>[2x]MLLLTPGPTPIPERVQKALLRPMRGHLDPEVLRVNRAIQERLAALFDPGEGALVAALAGSGSLGM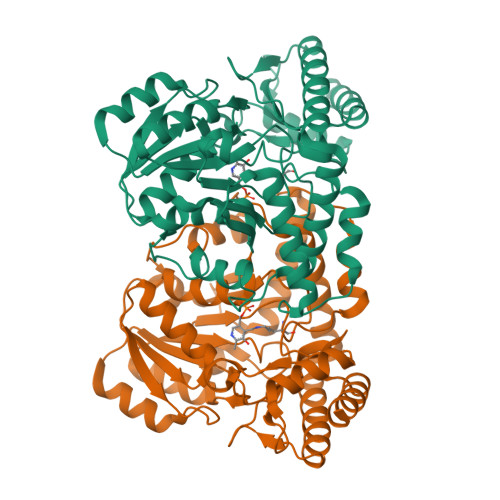EAGLANLDRGPVLVLVNGAFSQRVAEMAALHGLDPEVLDFPPGEPVDPEAVARALKRRRYRMVALVHGETSTGVLNPAEAIGALAKEAGALFFLDAVTTLGMLPFSMRAMGVDYAFTGSQKCLSAPPGLAPIAASLEARKAFTGKRGWYLDLARVAEHWERGGYHHTTPVLLHYALLEALDLVLEEGVAARERRAREVYAWVLEELKARGFRPYPKASPLPTVLVVRPPEGVDADRLVRALYAEGVAVAGGIGPTRGQVLRLGLMGEGARREAYQAFLKALDRALALA> 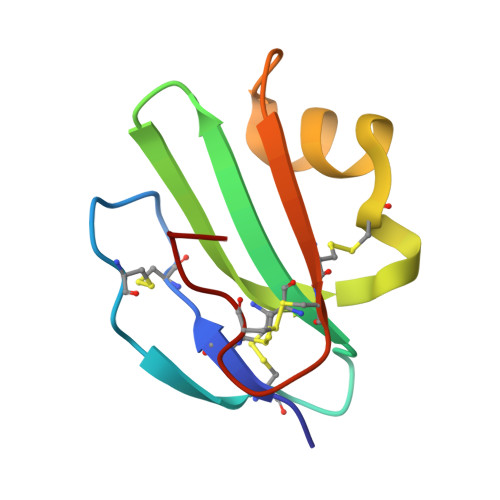FLQCYNCPNPTADCKTAVQCSSDFDACLITKAGLQVYNKCWKFEHCNFNDVTTRLRENELTYYCCKKDLCNFNEQ> IQE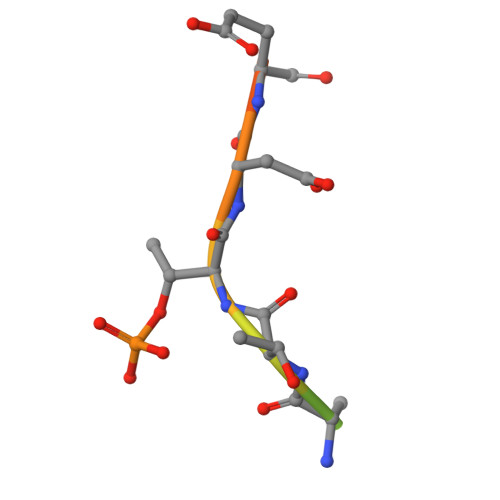LDSTTDEDEI> M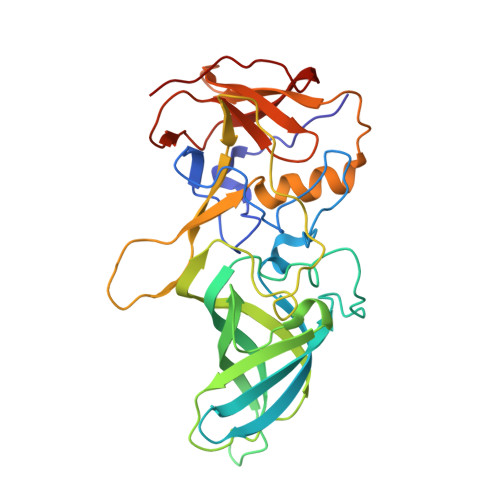VDLPVIQPRLCTHARWPAPVYGLLVDPSLPSNPQWQNGRVHVDGTLLGTTPISGSWVSCFAAEAAYKFQSGTGEVATFTLIEQDGSAYVPGDRAAPLGYPDFSGQLEIEVQTETTKTGDKLKVTTFEMILGPTTNADQAPYQGRVFASVTAAASLDLVDGRVRAVPRSIYGFQDTIPEYNDGLLVPLAPPIGPFLPGEVLLRFRTYMRQIDTADAAAEAIDCALPQEFVSWFASNAFTVQSEALLLRYRNTLTGQLLFECKLYNEGYIALSYSGSGPLTFPTDGIFEVVSWVPRLYQLASVGS>[4x]MELLQGKTFVVMGVANQRSIAWGIARSLHNAGAKLIFTYAGERLERNVRELA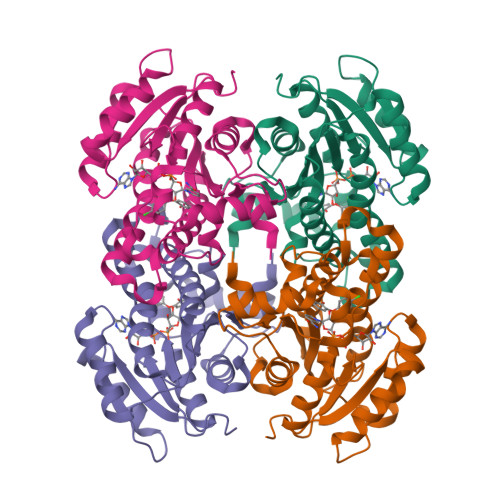DTLEGQESLVLPCDVTNDEELTACFETIKQEVGTIHGVAHCIAFANRDDLKGEFVDTSRDGFLLAQNISAFSLTAVAREAKKVMTEGGNILTLTYLGGERVVKNYNVMGVAKASLEASVKYLANDLGQHGIRVNAISAGPIRTLSAKGVGDFNSILREIEERAPLRRTTTQEEVGDTAVFLFSDLARGVTGENIHVDSGYHILG> ACRPGATRMKWYFQKPYVRRVKSDFFRFPLLSQVTKQKIDWQYHHPRSGYEAACIFGPNTLEVTNLPMGKTCQYLQERLWRFFGKFGIVEQVRVLPHERDPYQTCGTAYVCFRSRMASLRAVRLPVHLPASLHNRVLHLRHLGTDRTSDDLFYFRRQQAISNLVAIAQQLYAYLEERGP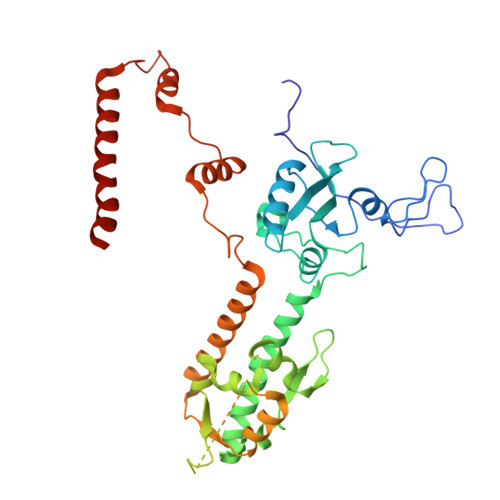LPAHRALRLLFERSYPRLAWRQAGVSVRTCCGSWLGFFSRSPFNELFYLAREDEVARPTEVTELEADPRASRKMISNEGTEGAAETRGRKTKSKLGDTKDGTSPGLKSLTDREENAMLEKMVIFPHLLSREKLQALLLRAGRLLQMDLQNELSVHWRTDRPPLPDWTQKQIQLWQHQDPLPEELQIWSRTKDYYKIHEERFLFKLKLKKERAQAKQEMKQQRRRLE> XVNAKQYHRILKRRQARAKLEAEGKIPKERX;> GPSFREQDIYLPIANVARIMKNAIPQTGKIAKDAKECVQECVSEFISFITSEASERCHQEKRKTINGEDILFAMSTLGFDSYVEPLKLYLQKFRE;> GPMEEIRNLTVKDFRVQELPLARIKKIMKLDEDVKMISAEAPVLFAKAAQIFITELTLRAWIHTEDNKRRTLQRNDIAMAITKFDQFDFLIDIVPR

Even though constrained helical interaction motifs generally show a tendency to inhibit PPIs,1a only very few have been reported to directly target transcription factors with sufficient affinity to enable the inhibition of complex assembly.12a, 14 The nuclear transcription factor Y (NF‐Y)15 is a trimeric complex (NF‐YA/B/C) that binds to a particular DNA sequence (CCAAT box), thereby activating genes involved in regulation of the cell cycle and DNA repair. NF‐Y subunits B and C form a stable heterodimer, which by itself does not possess relevant affinity to DNA target sequences (CCAAT box DNA). Only upon availability and binding of the third subunit (NF‐YA) is the transcriptionally active trimeric complex formed and DNA binding occurs with affinity values in the low nanomolar range. In this study, we aimed to inhibit the interaction between the NF‐YB/C heterodimer (light/dark grey) and NF‐YA (green) to prevent transcription‐factor assembly and DNA (blue) binding.

For PBM, we observe well‐defined electron density for all amino acids except G289 and R295, both located in the C‐terminal part of the peptide. The central part of PBM adopts an α‐helical conformation (Y272–A287), which is flanked by extended peptide stretches. Except for the C‐terminal part (K290–E294), PBM superimposes closely with NF‐YA in the DNA‐bound complex (RMSD for V267–E288: 0.52 Å). To identify the crucial interaction motif within PBM, six truncated sequences (1–6) and PBM were synthesized and fluorescently labeled to determine dissociation constants with the NF‐YB/C dimer using a fluorescence polarization (FP) assay. Initially, we identified a 14‐mer α‐helix with a short extended N‐terminal stretch as the protein fragment crucial for NF‐YB/C binding.> NQNEALLQAIKARNIRLSEAACEDEDSASEGLGELFLDGLSTENPHGARLSLDGQGRLS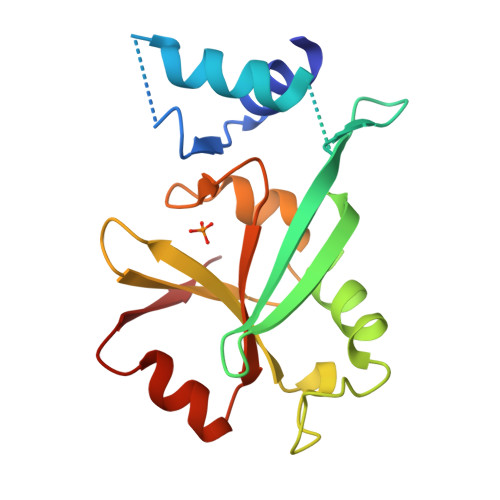WPVLFLYPEYAQSDFISAFHEDSRFIDHLMVMFGETPSWDLEQKYCPDNLEVYFEDEDRAELYRVPAKSTLLQVLQHQRYFVKALTPAFLVCVGSSPFCKNFLRGRKVYQIR> MGWDLTVKMLAGNEFQVSLSSSMSVSELKAQITQKIGVHAFQQRLAVHPSGVALQDRVPLASQGLGPGSTVLLVVDKSDEPLSILVRNNKGRSSTYEVRLTQTVAHLKQ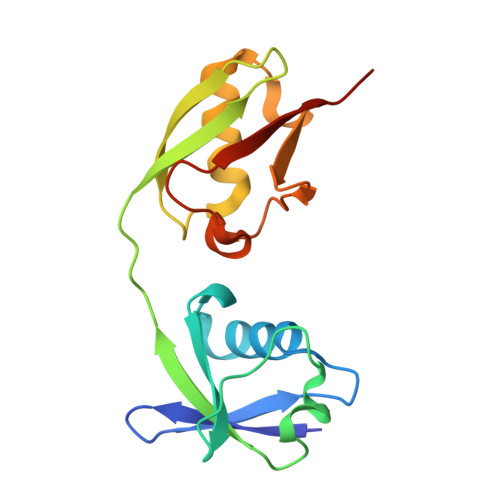QVSGLEGVQDDLFWLTFEGKPLEDQLPLGEYGLKPLSTVFMNLRLRGGGR> MASNQQQKEDPKEQQQQYKTFMGARVLWPPECADDILEGAIRETQDALKKFEIAREGQKIAEHLKKYMDDHFDPYW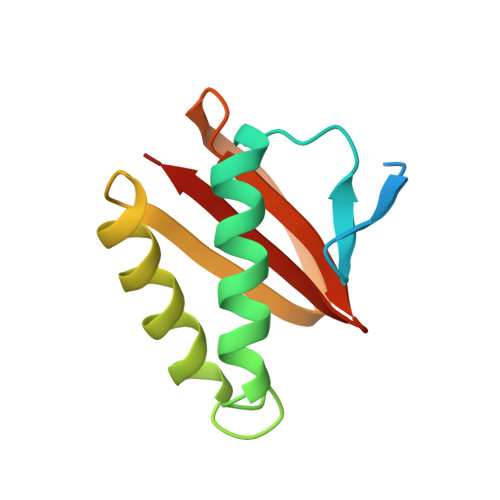HVFFGKNFGCQAVHNKNRFIYFYIEKTAFLMYQTQ> MHHHHHHGSPIFLNVLEAIEPGVVCAGHDNNQPDSFAALLSSLNELGERQLVHVVKWAKALPGFRNLHVDDQMAVI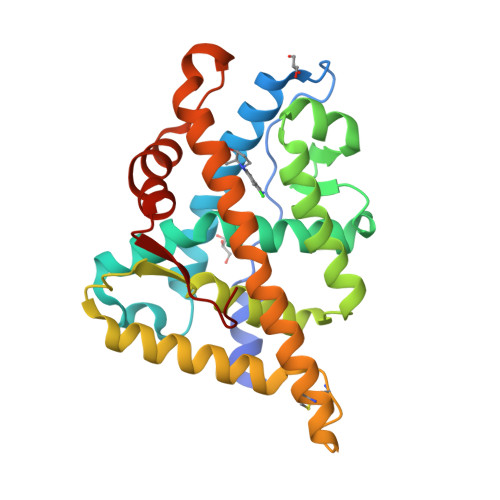QYSWMGLMVFAMGWRSFTNVNSRMLYFAPDLVFNEYRMHKSRMYSQCVRMRHLSQEFGWLQITPQEFLCMKALLLFSIIPVDGLKNQKFFDELRMNYIKELDRIIACKRKNPTSCSRRFYQLTKLLDSVQPIARELHQFTFDLLIKSHMVSVDFPEMMAEIISVQVPKILSGKVKPIYFHTQ> MAASSSGEKEKERLGGGLGVAGGNSTRERLLSALEDLEVLSRELIEMLAISRNQKLLQAGEENQVLELLIHRDGEFQELMKLALNQGKIHHEMQVLEKEVEKRDSDIQQLQKQLKEAEQILATAVYQAKEKLKSIEKARKGAISSEEIIKYAHRISASNAVCAPLTWVPGDPRRPYPTDLEMRSGLLGQMNNPSTNGVNGHLPGDALAAGRLPDVLAPQYPWQSNDMS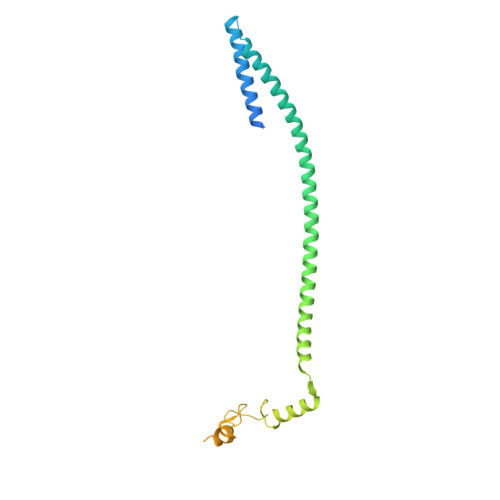MNMLPPNHSSDFLLEPPGHNKENEDDVEIMSTDSSSSSSESD> MVLPRLIPRLSRSAFKVAQANNRV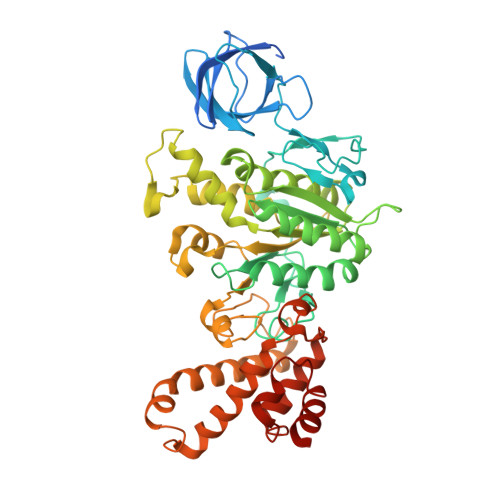FNAPFRGMASSAGVGSGKIRTVIGAVVDVQFEQDNLPAILNALTIDRGEGNKLVLEVAQHLGENTVRTIAMDGTEGLVRGTSVADTGAPITIPVGRGTLGRIINVCGEPIDERGPIEATKFLPIHADPPTFAEQSTTAEVLETGIKVVDLLAPYARGGKIGLFGGAGVGKTVFIQELINNIAKAHGGFSVFCGVGERTREGNDLYREMKETGVINLEGESKVTLVFGQMNEPPGARARVALTGLTIAEYFRDEEGQDVLLFVDNIFRFTQAGSEVSALLGRIPSAVGYQPTLATDMGALQERITTTQKGSVTSVQAVYVPADDLTDPAPATTFAHLDATTVLSRGISELGIYPAVDPLDSKSRLLDIDVVGQEHYDVASNVQQTLQAYKSLQDIIAILGMDELSEQDKLTVERARKIQRFLSQPFTVAEVFTGIEGRLVSLKDTVRSFKEILDGKHDALPEAAFYMVGGIEEVVAKAEKLAAESK> MPEPHAVLYVTNELSHIVKDGFLPIWKLTGDESLNDLWLENGKYATDVYAYGDVSKWTIRQLRGHGFIFISTHKNVQLADIIKTVDVRIPREVARSHDMKAFENEIGRRRIRMRKGFGDALRNYAFKMAIEFHGSEAETLNDANPRLHKIYGMPEIPPLYMEYAEIGTRFDDEPTDEKLVSMLDYIVYSAEEVHYIGCGDLRTLMQFKKRSPGRFRRVLWHVYDPIAPECSDPNVIVHNIMVDSKKDILKHMNFLKRVERLFIWDVSSDRSQMNDHEWETTRFAEDRLGEEIAYEMGGAFSSALIKHRIPNSKDEYHCISTYLFPQPGADADMYELRNFMRLRGYSHVDRHMHPDASVTKVVSRDVRKMVELYHGRDRGRFLKKRLFEHLHIVRKNGLLHESDEPRADLFYLTNRCNMGLEPSIYEVMKKSVIATAWVGRAPLYDYDDFALPRSTVMLNGSYRDIRILDGNGAILFLMWRYPDIVKKDLTYDPAWAMNFAVSLKEPIPDPPVPDISLCRFIGLRVESSVLRVRNPTLHETADELKRMGLDLSGHLYVTLMSGAYVTDLFWWFKMILDWSAQNREQKLRDLKRSAAEVIEWKEQMAERPWHVRNDLIAAL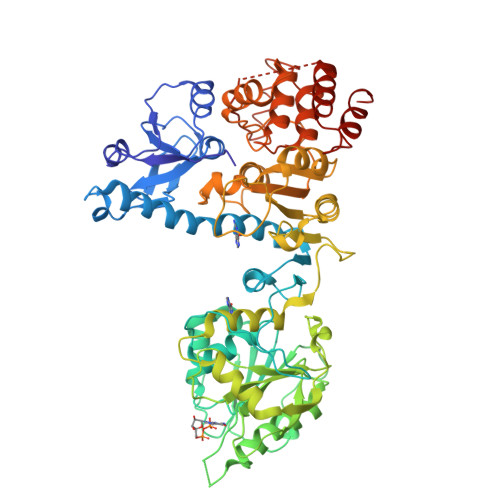REYKRKMGMREGASIDSWLELLRHL>DIFEAQKIEWHEGAHMT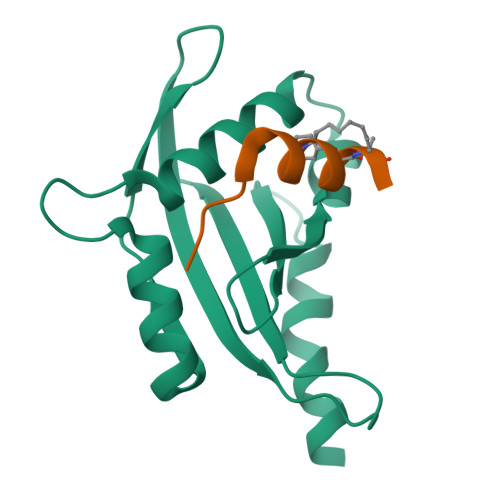GVESFMTKQDTTGKIISIDTSSLRAAGRTGWEDLVRKCIYAFFQPQGREPSYARQLFQEVMTRGTASSPSYRFILNDGTMLSAHTKCKLCYPQSPDMQPFIMGIHIIDRE[2x];>[2x]LLPPTEQDLLKLALYX>[10x]PGSIPLIGERFPEMEVTTDHGVIKLPDHYVSQGKWFVLFSHPADFTPVSTTEFVSFARRYEDFQRLGVDLIGL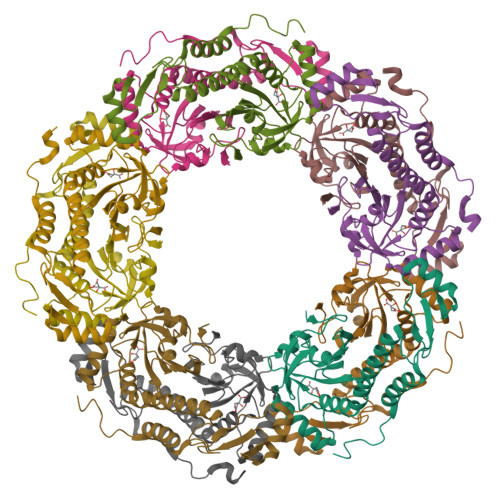SVDSVASHIKWKEWIERHIGVRIPFPIIADPQGTVARRLGLLHAESATHTVRGVFIVDARGVIRTMLYYPMELGRLVDEILRIVKALKLGDSLKRAVPADWPNNEIIGEGLIVPPPTTEDQARARMESGQYRSLDWWFSWDTPASRDDVEEARRYLRRAAEKPAKLLYEEA pyrene-1,3,6,8-tetrasulfonic 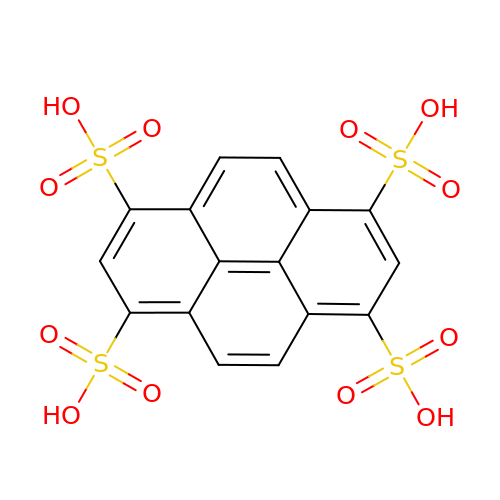acid | C16 H10 O12 S4 | CZLSHVQVNDDHDQ-UHFFFAOYSA-N>AMGIKHLNLTVADVVAAREFLEKYFGLTCSGTRGNAFAVMRDNDGFILTLMKGKEVQYPKTFHVGFPQESEEQVDKINQRLKEDGF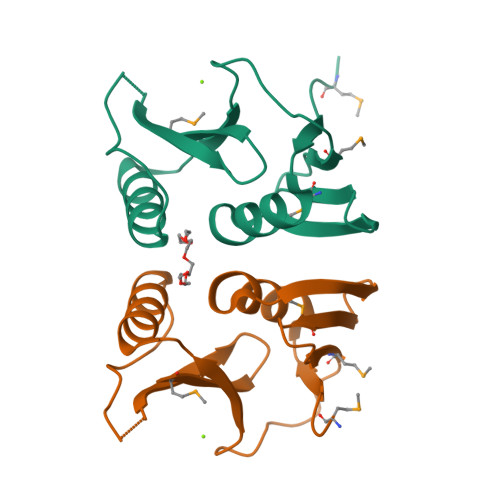LVEPPKHAHAYTFYVEAPGGFTIEVMC[2x]N'-{(1S,2R)-1-(3,5-DIFLUOROBENZYL)-2-HYDROXY-3-[(3-METHOXYBENZYL)AMINO]PROPYL}-5-METHYL-N,N-DIPROPYLISOPHTHALAMIDE 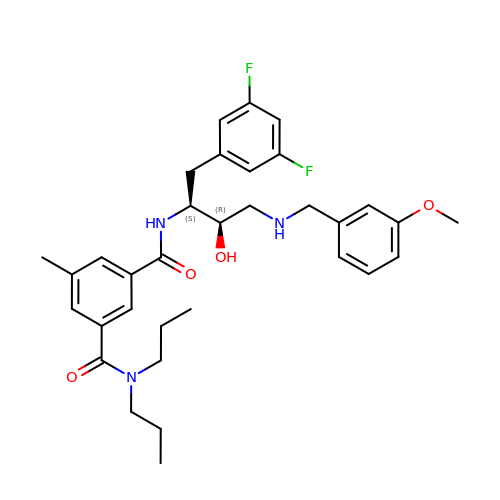| C33 H41 F2 N3 O4 | JEEOUWBWJFSMIP-IOWSJCHKSA-N> MAAASVTPPGSLELL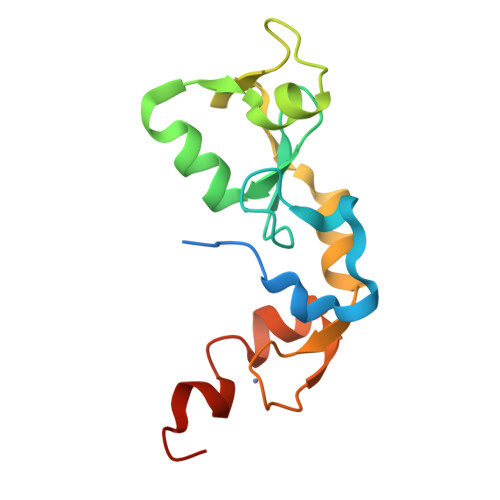QPGFSKTLLGTKLEAKYLCSACRNVLRRPFQAQCGHRYCSFCLASILSSGPQNCAACVHEGIYEEGISILESSSAFPDNAARREVESLPAVCPSDGCTWKGTLKEYESCHEGRCPLMLLEHHHHHH> ADLGSKNLKSPQKVEVDIIDDNFILRWNRSDESVGNVTFSFDYQKTGMDNWIKLSGCQNITSTKCNFSSLKLNVYEEIKLRIRAEKENTSSWYEVDSFTPFRKAQIGPPEVHLEAEDKAIVIHISPGTKDSVMWALDGLSFTYSLVIWKNSSGVEERIENIYSRHKIYKLSPETTYCLKVKAALLTSWKIGVYSPVHCIKTTVENELPPPENIEVSVQNQNYVLKWDYTYANMTFQVQWLHAFLKRNPGNHLYKWKQIPDCENVKTTQCVFPQNVFQKGIYLLRVQASDGNNTSFWSEEIKFDTEIQAFLLPPVFNIRSLSDSFHIYIGAPKQSGNTPVIQDYPLIYEIIFWENTSNAERKIIEKKTDVTVPNLKPLTVYCVKARAHTMDEKLNKSSVFSDAVCEKTKPGNTSK;> MCDLPQTHSLGSRRTLMLLAQMRRISLFSCLKDRHDFGFPQEEFGNQFQKAETIPVLYNMISQIFNLFSTKDSSAAWDETLLDKFYTELYQQLNDLEACVIQGVGVTETPLMKEDSILAVRKYFQRITLYLKEKKYSPCAWEVVRAEIMRSFSLSTNLQESLRSKE;> YTDESCTFKISLRNFRSILSWELKNHSIVPTHYTLLYTIMSKPEDLKVVKNCANTTRSFCDLTDEWRSTHEAYVTVLEGFS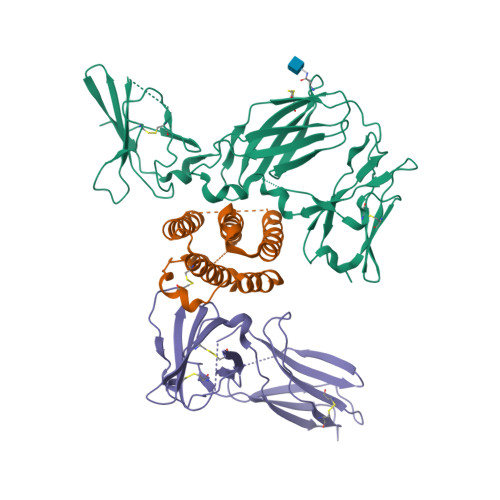GNTTLFSCSHNFWLAIDMSFEPPEFEIVGFTNHINVMVKFPSIVEEELQFDLSLVIEEQSEGIVKKHKPEIKGNMSGNFTYIIDKLIPNTNYCVSVYLEHSDEQAVIKSPLKCTLLPP> MKNKLGVFVVCLFCQIMLGQNGTRKSLHGQVTNKSLAIESGYVMNINAKSRTFIGPGGLFDILAQPKDTLLFTGIAFQSKKIVLTEKDCSQILFSVSLDLVSNELKEVLVRKDLKVK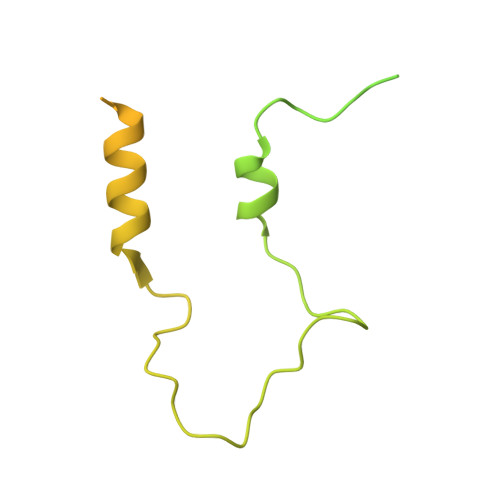SLDSNTQKYVDMQFEDDRQSTAKNTVMYSDQTIKYGTDFVRIFKDVKKLLSKNNEKEEVISDIAFVEYSKANFKPDFYTKTLGLKPDEVDLFLMFCSNDPESKRHLNEDQKFELIDFLINKNAEFKKVNAAQ>[2x]MVSEMLEEIKRTIMQRLPERVQVAKVEFEGPEVVIYTKNPEIITENGNLIRDIAKDIRKRIIIRSDRSVLMDPEKAIRKIHEIVPEEAKITNISFDDVTCEVIIEARKPGLVIGKYGSTSREIVKNTGWAPKILRTPPISSEIIERIRRTLRKNSKERKKILQQLGNRIHQKPKYDNDWARLTAMGGFREVGRSCLYLQTPNSRVLLDCGVNVAGGDDKNSYPYLNVPEFTLDSLDAVIITHAHLDHSGFLPYLYHYGYDGPVYCTAPTRDLMTLLQLDHIDIAHREDEPLPFNVKHVKKSVKHTITLDYGEVTDIAPDIRLTLHNAGHILGSAMAHLHIGDGQHNMVYTGDFKYEQSRLLEAAANRFPRIETLVMESTYGGHEDVQPSRNRAEKELVKTIYSTLRRGGKILIPVFAVGRAQELMIVLEEYIRTGIIDEVPVYIDGMIWEANAIHTARPEYLSKDLRDQIFHMGHNPFISDIFHKVNGMDERREIVEGEPSIILSTSGMLTGGNSLEYFKWLCEDPDNSLVFVGYQAEGSLGRRIQKGWKEIPLKDEDDKMRVYNVRMNIKTIEGFSGHSDRRQLMEYVKRISPKPEKILLCHGDNYKTLDLASSIYRTYRIETKTPLNLETVRIQ

MTH1203, a β-CASP metallo-β-lactamase family nuclease from the archaeon Methanothermobacter thermautotrophicus, was identified as a putative nuclease that might contribute to RNA processing. The crystal structure of MTH1203 reveals that, in addition to the metallo-β-lactamase nuclease and the β-CASP domains, it contains two contiguous KH domains that are unique to MTH1203 and its orthologs. In vitro nuclease activity assays demonstrated that MTH1203 is a zinc-dependent nuclease. MTH1203 is also shown to be a dimer and, significantly, this dimerization enhances the nuclease activity.

The MTH1203 crystal structure was solved by molecular replacement at a resolution of 3.1 Å, using X-ray data collected at the zinc absorption peak. The MTH1203 protein has a tripartite architecture consisting of the two N-terminal KH domains (KHa and KHb), the central MBL domain and the C-terminal β-CASP domain. The two molecules found in the asymmetric unit are essentially identical and superpose with a root mean square deviation of 0.65 Å. Two zinc ions are observed in the active site which is situated at the bottom of a cleft in the MBL domain. The two zinc atoms are coordinated in an octahedral geometry by the bound phosphate and the conserved residues His242, His244, Asp246, and His247 from motif 2, His329 (motif 3), Asp352 (motif 4), His579 (motif B), and His603 (motif C) located in the MBL domain, similar to the active site structures of CPSF-73 and TTHA0252. A phosphate group present in the active site is a good mimic for the phosphate group of a nucleotide ready to be hydrolysed. The N-terminal KH domain (KHa, residues 1–70) was not detected by sequence analysis because it lacks the signature GXXG motif. However, this domain lacks the GXXG motif that is essential for RNA binding (Lin et al., 1997; Siomi et al., 1994), and the conformation of its helix-turn-helix structure, crucial for RNA binding, is different suggesting that the KHa domain does not bind RNA. Interestingly, the RNA-binding site of KHb is distant to the active site of the MBL domain, being separated by ∼42 Å with no significant positively charged regions observed on the molecular surface between the two domains. Analysis of MTH1203 using PISA indicates that MTH1203 forms a stable dimer in solution. This assembly, with a protein-protein interface area of 933 Å2, involves a symmetrical interaction between the C terminus region of each monomer, a loop and a β strand from the MBL domain.>[2x]SCPHVALLLSSGMGHLTPCLRFAATLVQHHCRVTIITNYPTVSVAESRAISLLLSDFPQITEKQFHLLPFDPSTANTTDPFFLRWEAIRRSAHLLNPLLSSISPPLSALVIDSPLVSSFVPVAANLDLPSYVLFTSSTRMCSLQETFPAFVASKTNFDSIQLDDVIEIPGFSPVPVSSVPPDFLNLNHLFTTMLIQNGQSFR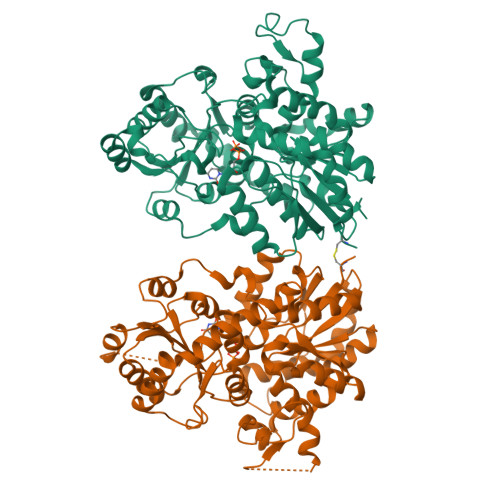KANGILINTFEALEGGILPGINDKRAADGLPPYCSVGPLLPCKFEKTECSAPVKWLDDQPEGSVVYVSFGSRFALSSEQIKELGDGLIRSGCRFLWVVKCKKVDQEDEESLDELLGRDVLEKIKKYGFVIKNWVNQQEILDHRAVGGFVTHGGWNSSMEAVWHGVPMLVWPQFGDQKINAEVIERSGLGMWVKRWGWGTQQLVKGEEIGERIKDLMGNNPLRVRAKTLREEARKAIEVGGSSEKTLKELIENWKKTSRKT> GPDSMADAFGDELFSVFEGDSTTAAGTKKDKEKDKGKWKGPPGSADKAGKRFDGKLQSESTNNGKNKRDVDFEGTDEPIFGKKPRIEESITEDLSLADLMPRVKVQSVETVEGCTHEVALPAEEDYLPLKPRVGKAAKEYPFILDAFQREAIQCVDNNQSVLVSAHTSAGKTVCAEYAIALALREKQRVIFTSPIKALSNQKYREMYEEFQDVGLMTGDVTINPTASCLVMTTEILRSMLYRGSEVMREVAWVIFDEIHYMRDSERGVVWEETIILLPDNVHYVFLSATIPNARQFAEWICHLHKQPCHVIYTDYRPTPLQHYIFPAGGDGLHLVVDENGDFREDNFNTAMQVLRDAGDLAKGDQKGRKGGTKGPSNVFKIVKMIMERNFQPVIIFSFSKKDCEAYALQMTKLDFNTDEEKKMVEEVFSNAIDCLSDEDKKLPQVEHVLPLLKRGIGIHHGGLLPILKETIEILFSEGLIKALFATETFAMGINMPARTVLFTNARKFDGKDFRWISSGEYIQMSGRAGRRGMDDRGIVILMVDEKMSPTIGKQLLKGSADPLNSAFHLTYNMVLNLLRVEEINPEYMLEKSFYQFQHYRAIPGVVEKVKNSEEQYNKIVIPNEESVVIYYKIRQQLAKLGKEIEEYIHKPKYCLPFLQPGRLVKVKNEGDDFGWGVVVNFSKKSNVKPNSGELDPLYVVEVLLRCSKESLKNSATEAAKPAKPDEKGEMQVVPVLVHLLSAISSVRLYIPKDLRPVDNRQSVLKSIQEVQKRFPDGIPLLDPIDDMGIQDQGLKKVIQKVEAFEHRMYSH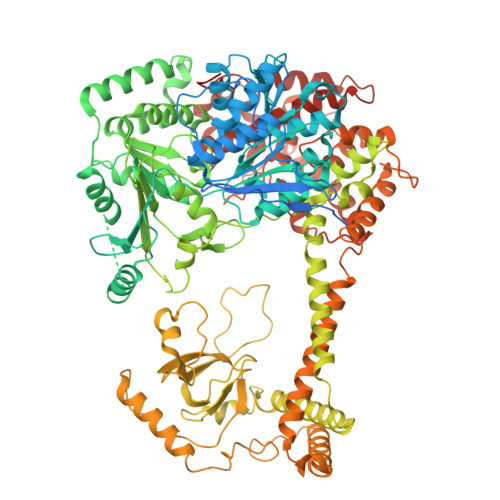PLHNDPNLETVYTLCEKKAQIAIDIKSAKRELKKARTVLQMDELKCRKRVLRRLGFATSSDVIEMKGRVACEISSADELLLTEMMFNGLFNDLSAEQATALLSCFVFQENSSEMPKLTEQLAGPLRQMQECAKRIAKVSAEAKLEIDEETYLSSFKPHLMDVVYTWATGATFAHICKMTDVFEGSIIRCMRRLEELLRQMCQAAKAIGNTELENKFAEGITKIKRDIVFAASLYL> SVIGRIHSFESCGTVDGPGIRFITFFQGCLMRCLYCHNRDTWDTHGGKEVTVEDLMKEVVTYRHFMNASGGGVTASGGEAILQAEFVRDWFRACKKEGIHTCLDTNGFVRRYDPVIDELLEVTDLVMLDLKQMNDEIHQNLVGVSNHRTLEFAKYLANKNVKVWIRYVVVPGWSDDDDSAHRLGEFTRDMGNVEKIELLPYHELG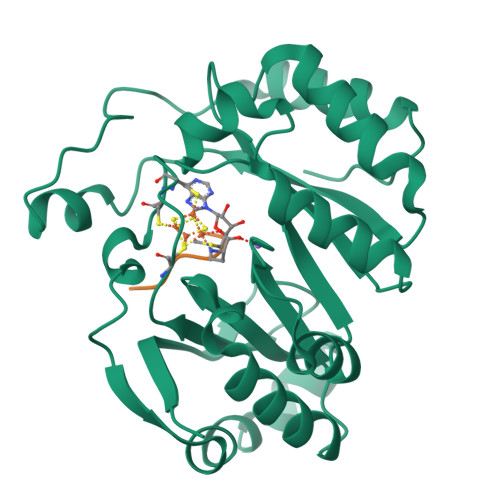KHKWVAMGEEYKLDGVKPPKKETMERVKGILEQYGHKVMF;> VSGYAV>[2x]AERPPEETLSLWKGEQARLKARVVDRDTEAWQRDPSFSGLQKVGGVDVSFVKGDSVRACASLVVLSYPELKVVYEDSRMVGL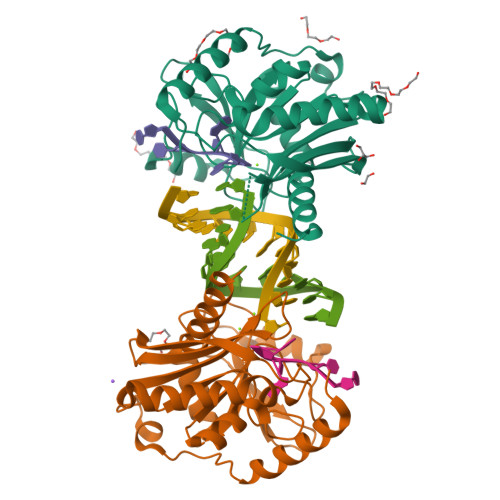KAPYVSGFLAFREVPFLVELVQRLQEKEPDLMPQVVLVDGNGVLHQRGFGVACHLGVLTELPCIGVAKKLLQVDGLENNALHKEKIVLLQAGGDTFPLIGSSGTVLGMALRSHDHSTKPLYVSVGHRISLEVAVRLTHHCCRFRIPEPIRQADIRSREYIRRTLG>GPLGSDNKVLHVYNWSDYIAPDTLEKFTKETGIKVVYDVYDSNEVLEAKLLAGKSGYDVVVPSNSFLAKQIKAGVYQKLDKSKLPNWKNLNKDLMHTLEVSDPGNEHAIPYMWGTIGIGYNPDKVKAAFGDNAPVDSWDLVFKPENIQKLKQCGVSFLDSPTEILPAALHYLGYKPDTDNPKELKAAEELFLKIRPYVTYFHSSKYISDLANGNICVAIGYSGDIYQAKSRAEEAKNKVTVKYNIPKEGAGSFFDMVAIPKDAENTEGALAFVNFLMKPEIMAEITDVVQFPNGNAAATPLVSEAIRNDPGIYPSEEVMKKLYTFPDLPAKTQRAMTRSWTK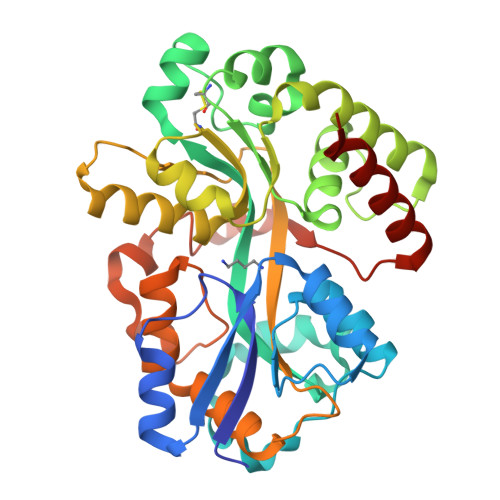IKSG[2x]> MSLVNRKQLEKMANVRFRTQEDEYVAILDALEEYHNMSENTVVEKYLKLKDINSLTDICIDTYKKSGRNKALKKFKEYLVTEVLELKNNNLTPVEKNLHFVWIGGQINDTAINYINQWKDVNSDYNVNVFYDSNAFLINTLKKTVVESAINDTLESFRENLNDPRFDYNKFFRKRMEIIYDKQKNFINYYKAQREENPELIIDDIVKTYLSNEYSKEIDELNTYIEESLNKITQNSGNDVRNFGEFKNGESFNLYEQELVERWNLAAASDILRISALKEIGGMYLDVDMLPGIQPDLFESIEKPSSVTVDFWEMTKLEAIMKYKEYIPEYTSEHFDMLDEEVQSSFESVLASKSDKSEIFSSLGDMEASPLEVKIAFNSKGIINQGLISVKDSYCSNLIVKQIENRYKILNNSLNPAISEDNDFNTTTNTFIDSIMAEANADNGRFMMELGKYLRVGFFPDVKTTINLSGPEAYAAAYQDLLMFKEGSMNIHLIEADLRNFEISKTNISQSTEQEMASLWSF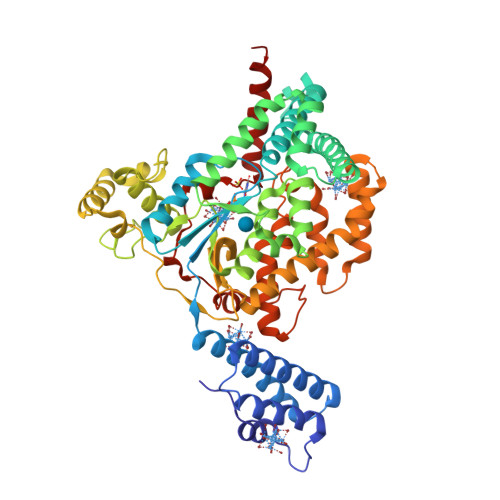DDARAKAQFEEYKRNYFEGAL>MAHHHHHHVGTFENITAAPADPILGLADLFRADERPGKVDLGVGVYKDETGKTPVMTSVKKAEQYLLENETTKTYLGIDGIPEFGRCTQELLFGKGSALINDKRARTAQTPGGSGALRVAADFLAKNTSVKRVWVSNPTWPNHKAIFNSAGLEVREYAYYDAENHTLDFDALINSLNEAQAGDVVLFHGCCHNPTGIDPTLEQWQTLAQLSVEKGWLPLIDIAYQGFGRGLEEDAEGLRAFAAMHKELIVASSCSKNFSLYNERVGACTLVAADSETVDRAFSQMKAAIRANYSS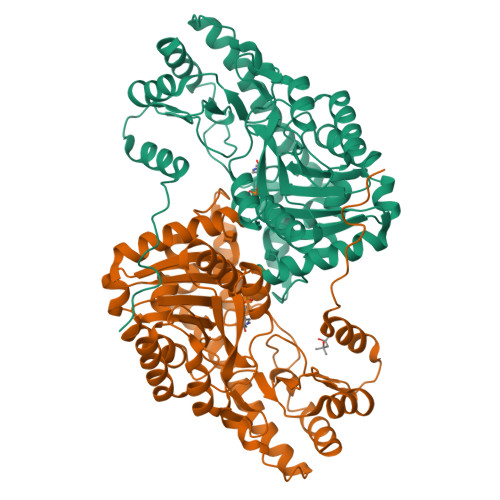PPAHGASVVATILSNDALRAIWEQELTDMRQRIQRMRQLFVNTLQEKGANRDFSFIIKQNGMFSFSGLTKEQVLRLREEFGVYAVASGRINVAGMTPDNMAPLCEAIVAVL[2x]> MEDIIVVALYDYVSWSPDDLSFQKGDQMVVLEESGEWWKARSLATRKEGYIPSNYVARVD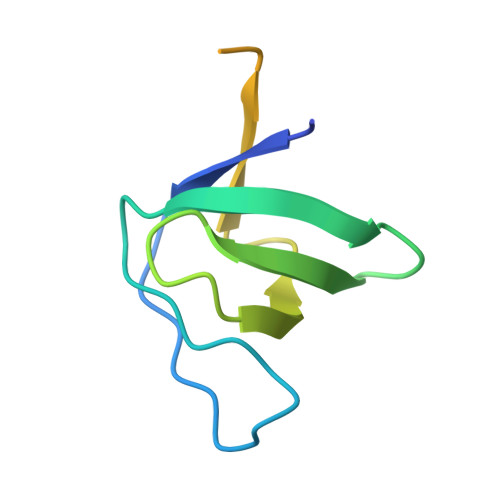SGGGTSGGGRHRRRQAERMSQIKRLLSEKK> MIITVTLNMEKYNFLGISIVGQSNERGDGGIYIGSIMKGGA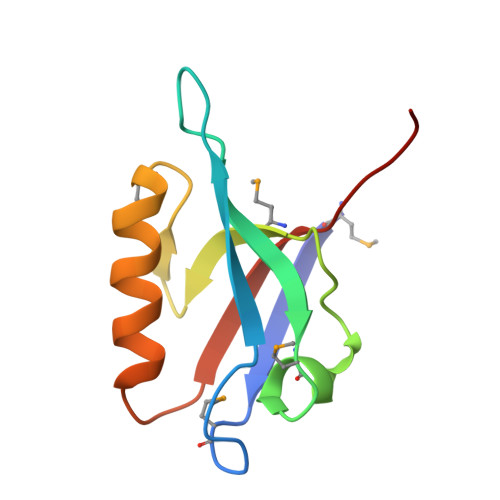VAADGRIEPGDMLLQVNDINFENMSNDDAVRVLRDIVHKPGPIVLTVAKLEHHH N-{3-[5-(1H-1,2,4-triazol-3-yl)-1H-indazol-3-yl]phenyl}furan-2-carboxamide 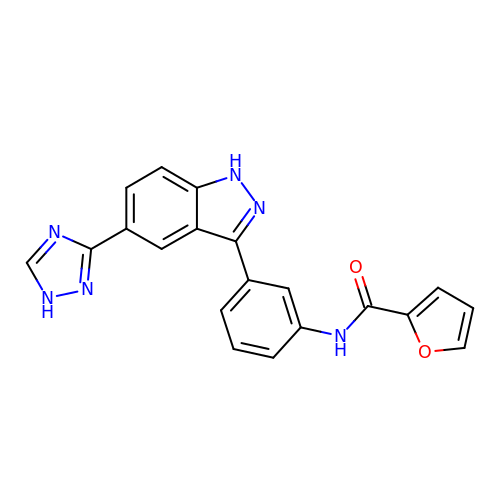| C20 H14 N6 O2 | LMDMJDCLPIVGQD-UHFFFAOYSA-N>PPYTVVYFPVRGRCAALRMLLADQGQSWKEEVVTVETWQEGSLKASCLYGQLPKFQDGDLTLYQSNTILRHLGRTLGLYGKDQQEAALVDMVNDGVEDLRCKYISLIYTNYEAGKDDYVKALPGQLKPFETLLSQNQGGKTFI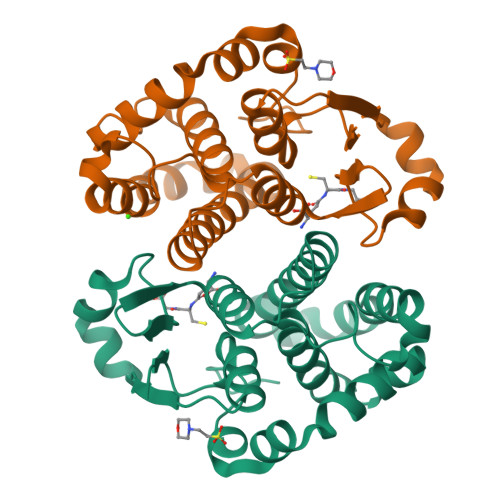VGDQISFAEYNLLDLLLIHEVLAPGCLDAFPLLSAYVGRLSARPKLKAFLASPEYVNLPINGNGKQ[2x]>MHHHHHHGSKKRIFIGSSSEQLTILNEIVDLLGDDVECIPWTDAFALNKSGLDSLIKQTRLADYSILIATKDDLTKQRGESLTKPRDNVVFEFGLFLGAAGPEKCYLIAEEDTDLPTDLDGITVAKFTRNSGQYNSLDKIVESIRTHLVKIAEMSQLGLLPSTALAIGYYNSFIKRVCEEIHGSECVELEGKKIKVKSFRVDVVIPETLDDNGVGNFTTLYNKRYGLSKATTCTNPALLGTRGFPFHFKVDPPDAN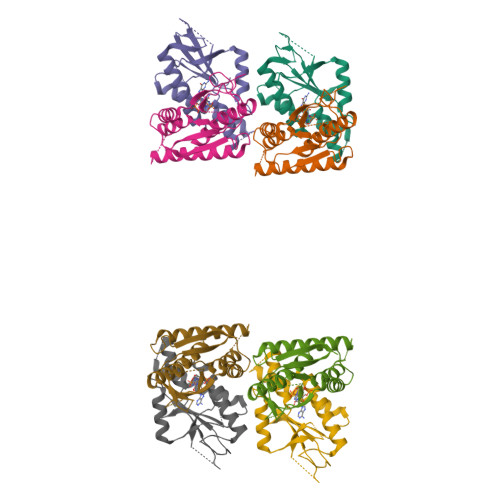QESPVDIHLLDIPSTLSTIVESLKLYLPSNQVGQDFDMDYLEMRELENFAKVLKYLIGRNAATKGYVNVLTNVKL[8x]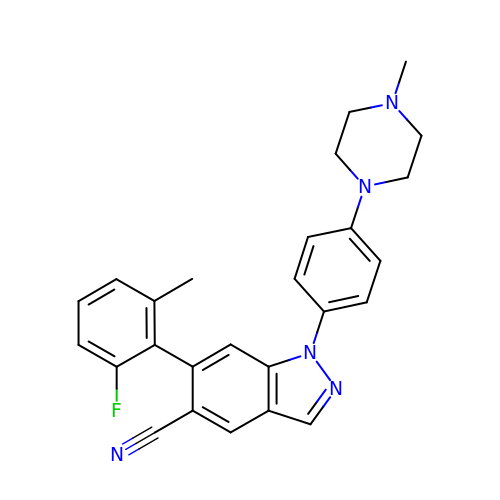6-(2-fluoro-6-methylphenyl)-1-[4-(4-methylpiperazin-1-yl)phenyl]-1H-indazole-5-carbonitrile | C26 H24 F N5 | YCDUCYZVJNKJTL-UHFFFAOYSA-N> AGGHGDVGMHVKEKEKNKDENKRKDEERNKTQEEHLKEIMKHIVKIEVKGEEAVKKEAAEKLLEKVPSDVLEMYKAIGGKIYIVDGDITKHISLEALSE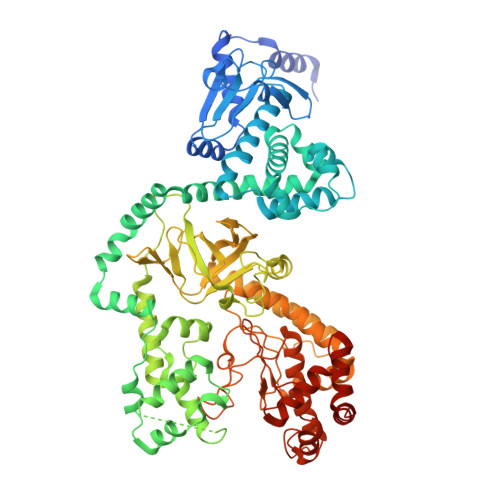DKKKIKDIYGKDALLHEHYVYAKEGYEPVLVIQSSEDYVENTEKALNVYYEIGKILSRDILSKINQPYQKFLDVLNTIKNASDSDGQDLLFTNQLKEHPTDFSVEFLEQNSNEVQEVFAKAFAYYIEPQHRDVLQLYAPEAFNYMDKFNEQEINLSLEELKDQRMLSRYEKWEKIKQHYQHWSDSLSEEGRGLLKKLQIPIEPKKDDIIHSLSQEEKELLKRIQIDSSDFLSTEEKEFLKKLQIDIRDSLSEEEKELLNRIQVDSSNPLSEKEKEFLKKLKLDIQPYDINQRLQDTGGLIDSPSINLDVRKQYKRDIQNIDALLHQSIGSTLYNKIYLYENMNINNLTATLGADLVDSTDNTKINRGIFNEFKKNFKYSISSNYMIVDINERPALDNERLKWRIQLSPDTRAGYLENGKLILQRNIGLEIKDVQIIKQSEKEYIRIDAKVVPKSKIDTKIQEAQLNINQEWNKALGLPKYTKLITFNVHNRYASNIVESAYLILNEWKNNIQSDLIKKVTNYLVDGNGRFVFTDITLPNIAEQYTHQDEIYEQVHSKGLYVPESRSILLHGPSKGVELRNDSEGFIHEFGHAVDDYAGYLLDKNQSDLVTNSKKFIDIFKEEGSNLTSYGRTNEAEFFAEAFRLMHSTDHAERLKVQKNAPKTFQFINDQIKFIINS> LSADQISTVQASFDKVKGDPVGILYAVFKADPSIMAKFTQFAGKDLESIKGTAPFETHANRIVGFFSKIIGELPNIEADVNTFVASHKPRGVTHDQLNNFRAGFVSYM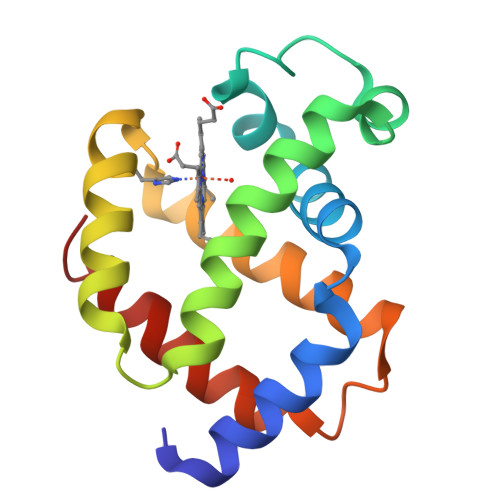KAHTDFAGAEAAWGATLDTFFGMIFSKM> MNLLIDNWIPVRPRNGGKVQIINLQSLYCSRDQWRLSLPRDDMELAALALLVCIGQIIAPAKDDVEFRHRIMNPLTEDEFQQLIAPWIDMFYLNHAEHPFMQTKGVKANDVTPMEKLLAGVSGATNCAFVNQPGQGEALCGGCTAIALFNQANQAPGFGGGFKSGLRGGTPVTTFVRGIDLRSTVLLNVLTLPRLQKQFPNESHTENQPTWIKPIKSNESIPASSIGFVRGLFWQPAHIELCDPIGIGKCSCCGQESNLRYTGFLKEKFTFTVNGLWPHPHSPCLVTVKKGEVEEKFLAFTTSAPSWTQISRVVVDKIIQNENGNRVAAVVNQFRNIAPQSPLELIMGGYRNNQASILERRHDVLMFNQGWQQY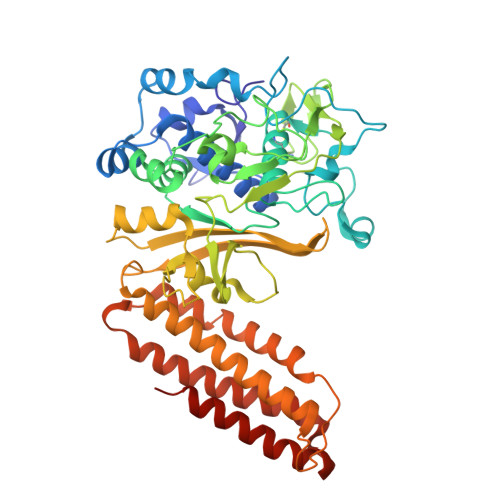GNVINEIVTVGLGYKTALRKALYTFAEGFKNKDFKGAGVSVHETAERHFYRQSELLIPDVLANVNFSQADEVIADLRDKLHQLCEMLFNQSVAPYAHHPKLISTLALARATLYKHLRELKPQGGPSNG bn7GpppG mRNA 5' cap analog | C27 H31 N10 O18 P3 | 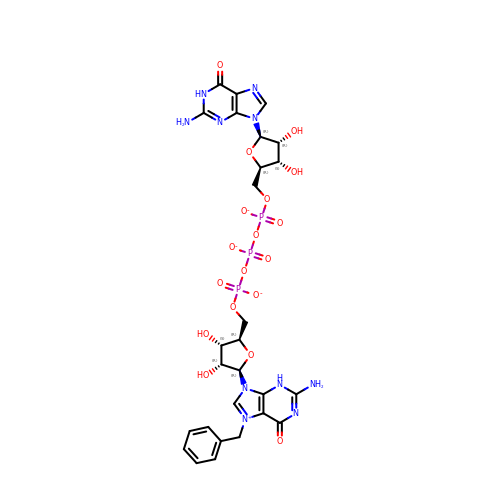DBIWUCQKTGTGGL-JIUDXVAXSA-L In the present study, a putative cell-wall lytic enzyme (EfAmi1) with predictive amidase activity was identified in the prophage sequence integrated into the Enterococcus faecium 11C6_DIV0699 genome and characterized. EfAmi1 is composed by two domains: a N-terminal Zn2+-dependent N-acetylmuramoyl-l-alanine amidase-2 (NALAA-2) domain and a C-terminal domain with unknown structure and function. The amidase-2 family includes Zn2+-dependent NALAAs that cleave the amide bond between N-acetylmuramic acid and L-Ala in bacterial cell walls. EfAmi1 exhibits broad-spectrum activity against both Gram-positive and Gram-negative bacteria.

The results revealed that only the catalytic amidase-2 domain (aa 2–185) was crystallized and its 3D structure was determined at 1.97 Å resolution. The absence of the C-terminal domain from the resolved structure was due to protein degradation, as discussed in another section. Analysis of the resolved structure revealed the presence of a β-sheet bundle structure, comprising of five β-strands: β1 (amino acids 3–6), β2 (amino acids 23–28), β3 (amino acids 57–60), β4 (amino acids 63–66), β5 (amino acids 86–91). The bundle is framed by four large α-helices (α1, α4, α6, α7) and 3 smaller ones (α2, α3, α5). This secondary structure forms a characteristic cavity in the middle of the structure. The presence of a zinc ion (Zn2+) was observed inside the cavity, although no Zn2+ was added to the crystallization buffer. The zinc ion in EfAmi1 structure is coordinated by two histidines (His27, His132) and a cysteine residue (Cys140), which are highly conserved. The tetrahedral coordination sphere of zinc is completed by a chloride ion. The architecture and size of the zinc-binding cavity indicates that it most likely serves as the binding site for the peptidoglycan. However, Thr330 in LysGH15 contributes to catalytic activity as revealed by the finding that the Thr330Ala mutant demonstrates a 50% decreased activity. Therefore, Glu90 and Thr138 are predicted to be key residues in EfAmi1.

> MVNIINNSVCRGVAGRRVGDVKGVVIHNTWTNTTAEQEMNRLAGMTDKQLEAGFAHYYCDENTIIRTEDTYNRAWHVANSDGNNSYIGYEVRGNRETPKAVFLQAEQNAFWQAAEDLRFYGLPVNRNTVKCHHQFSATECPKRSLMEHCGYDSTLAVPAAITVQMQDYFISQIKKYYDNPALKPDGSTEDQNHDDKVSASTPTHQGNAYGKLDIFKEVTDKTVRVAGWLVPDKPQGAIGTYAYVLVMEHGTPKELTRIQSQGIARPDVKKAYGYQGGDALGFDVTFDSSWMKGKKIDIILRRCNQSNGEGSVNDVRISDIYLILHHHHHH>SGIVP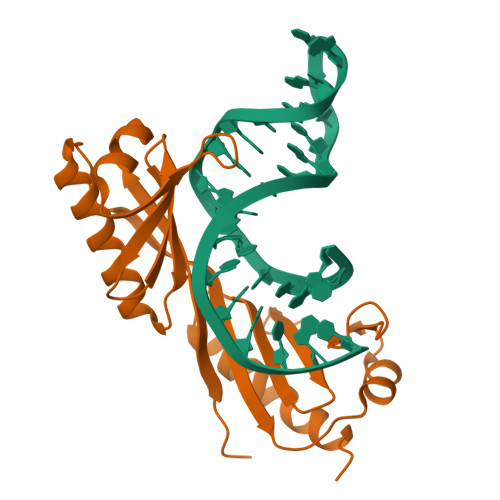TLQNIVATVTLGCRLDLKTVALHARNAEYNPKRFAAVIMRIREPKTTALIFASGKMVVTGAKSEDDSKLASRKYARIIQKIGFAAKFTDFKIQNIVGSCDVKFPIRLEGLAFSHGTFSSYEPELFPGLIYRMVKPKIVLLIFVSGKIVLTGAKQREEIYQAFEAIYPVLSEFRKM[2x]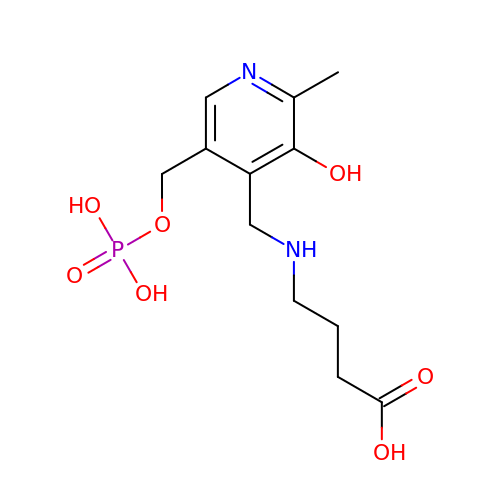4-[({3-HYDROXY-2-METHYL-5-[(PHOSPHONOOXY)METHYL]PYRIDIN-4-YL}METHYL)AMINO]BUTANOIC ACID | C12 H19 N2 O7 P | DOHWOHSLOVXAFH-UHFFFAOYSA-N>[2x]MGSHMEVNLRMSWWGGNGRHQVTLKALEEFHKQHPNINVKAEYTGWDGHLSRLTTQIAGGTEPDVMQTNWNWLPIFSK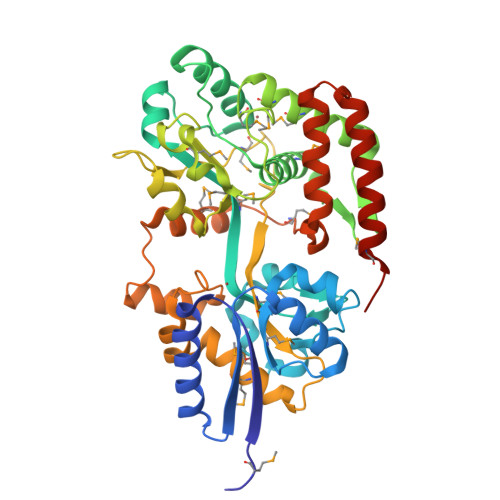DGTGFYNLFSVKEQLDLAQFDPKELQQTTVNGKLNGIPISVTAMIFYFNDATWAKAGLEYPKTWDELLAAGKVFKEKLGDQYYPVVLCAGQTLVLIRSYMTQKYNIPTIDEANKKFAYSPEQWVEFFTMYKTMVDNHVMPSTKYYASIVKSSYYEMKPWINGEWAGTYMWNSTITKYSDNLTKPAKLVLGPYPMLPGAKDAGLFFLPAQMLSIGKSTKHPQESAMLINFLLNSKEGVEALGLERGVPLSATAVTQLRASGVIKDEDPSVAGLNMALELPHPMTTSPYFLDWQIWSLFLDAIQYIDYGQKTVQETAEYFNKQGDRILKRAMRGSLEHHHHHH>[4x]MEKVAFIGLGAMGYPMAGHLARRFPTLVWNRTFEKALRHQEEFGSEAVPLERVAEARVIFTCLPTTREVYEVAEALYPYLREGTYWVDATSGEPEASRRLAERLREKGVTYLDAPVSGGTSGAEAGTLTVMLGGPEEAVERVRPFLAYAKKVVHVGPVGAGHAVKAINNALLAVNLWAAGEGLLALVKQGVSAEKALEVI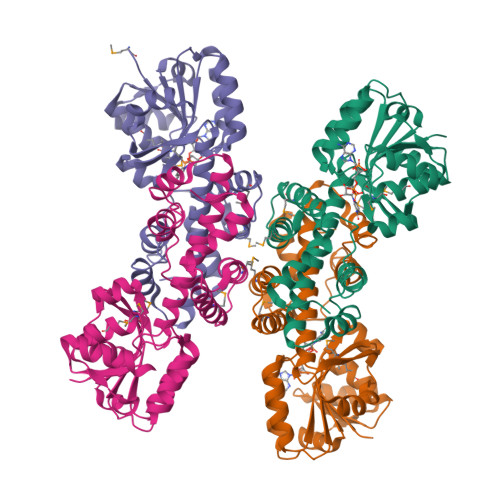NASSGRSNATENLIPQRVLTRAFPKTFALGLLVKDLGIAMGVLDGEKAPSPLLRLAREVYEMAKRELGPDADHVEALRLLERWGGVEIR> MATEKTEPTRANVEPPMPTRGASAWRRVRAWGPWLLGLSVAVRLAWAYLTPHGADLVDLHVYVSGPATLGHGNLYEFTYPDKTPDFPLPFTYPPFAAVVFWPLHLIPFTLLGLCWILGTIAALYAVVRLSQRLLGFDDARAAAVWTAVTMWTE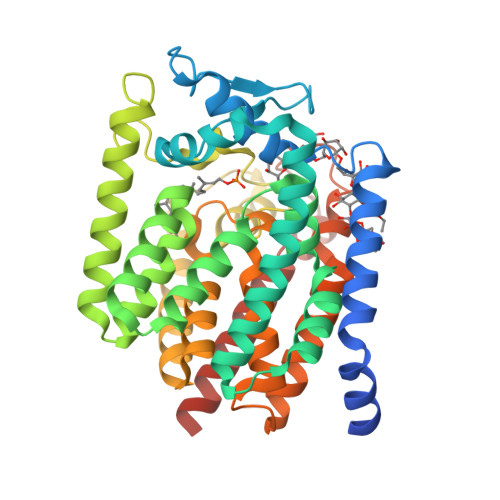PVRSTLDYGQINVLLMLLILLAVASSRWWISGTLIGLAGGVKLTPLVSGLYFLGARRWTTAIWAGVVFLLTVVVGIAVVGEQGRYYFTDLLGKPDRIGPIATVFNQSWRGGISRILGHDAGSGVLVLFAYAVTAILAFLAWRAVNDRLGQICVVEMFGLLISPISWTHHWVWMVPFMVWLLHGPWRDKVGAKVFGCGWLVLLLIGVPWLLSFAQPDIWRIDRPWPLAWAGLVDIVAAIATLTWMAVVGRRSGHLGRLPWRHV>GHMAFDLKTEDGLITYLTKHLSLDVDTSGVKRLSGGFVNVTWRIKLNAPYQGHTSIILKHAQPHMSTDEDFKIGVERSVYEYQAIKLMMANREVLGGVDGIVSVPEGLNYDLENNALIMQDVGKMKTLLDYVTAKPPLATDIARLVGTEIGGFVARLHNIGRERRDDPEFKFFSGNIVGRTTSDQLYQTIIPNAAKYGVDDPLLPTVVKDLVDDVMHSEETLVMADLWSGNILLQLEEGNPSKLQKIYILDWELCKYGPASLDLGYFLGDCYLISRFQDEQVGTTMRQAYLQSYARTSKHSINYAKVTAGIAAHIVMWTDFMQWGSEEERINFVKKGVAAFHDARGNNDNGEITSTLLKESSTA[2x]

Psilocybin, the natural hallucinogen from Psilocybe (magic) mushrooms, is a highly promising drug candidate for the treatment of depression and several other mental health conditions. Biosynthesis of psilocybin from the amino acid l‐tryptophan involves four strictly sequential modifications. The third of these, ATP‐dependent phosphorylation of the intermediate 4‐hydroxytryptamine, is catalysed by PsiK.

Here we present a crystallographic analysis and a structure‐based mutagenesis study of this kinase, providing insight into its mode of substrate recognition. The results of our work will support future bioengineering efforts aimed at generating variants of psilocybin with enhanced therapeutic properties.>[4x]MRKVSLALLLCLLCLAGMAQGQKALDLKDITSGRFRPENIQGVIPMPDGEHYTQMSADGTQIIKYSFRTGEKVEVIFDVNQARECDFKNFDSYQFSPDGDKLLIATRTTPIYRHSYTAVHYIYPLKRNDKGVTTNNIIERLSDGGPQQVPVFSPDGTMIAFVR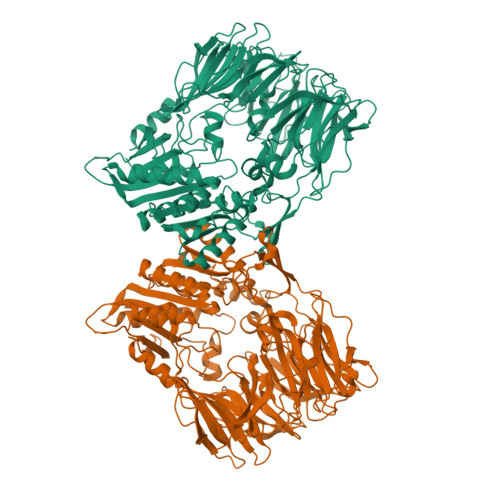DNNIFLVKLLYGNSESQVTEDGKQNSVLNGIPDWVYEEEFGFNRALEFSADNTMIAFIRFDESEVPSYSFPMFAGEAPQITPLKDYPGEYTYKYPKAGYPNSKVEVRTYDIKSHVTRTMKLPIDADGYIPRIRFTKDASKLAVMTLNRHQDRFDLYFADPRSTLCKLVLRDESPYYIKENVFDNIKFYPETFSLLSERDGFSHLYWYSMGGNLIKKVTNGKYEVKDFLGYDEADGSFYYTSNEESPLRKAVYKIDKKGKKLKLSQREGTNTPLFSQSMKYYMNKFSNLDTPMLVTLNDNTGKTLKTLINNDQLKQTLSGYAIPQKEFFTFQTTDGVTLNGWMMKPANFSTSKKYPVLMYQYSGPGSQQVLDTWGISWETYMASLGYIVVCVDGRGTGGRGEAFEKCTYLKIGVKEAKDQVETALYLGKQPYVDKDRIGIWGWSYGGYMTLMSMSEGTPVFKAGVAVAAPTDWRFYDTIYTERFMRTPKENAEGYKESSAFTRADKLHGNLLLVHGMADDNVHFQNCAEYAEHLVQLGKQFDMQVYTNRNHGIYGGNTRQHLYTRLTNFFLNNL> GPSSRWSKDYDVCVCHSEEDLVAAQDLVSYLEGSTASLRCFLQLRDATPGGAIVSELCQALSSSHCRVLLITPGFLQDPWCKYQMLQALTE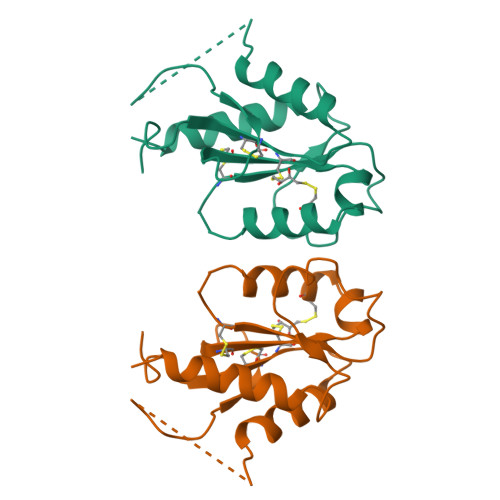APGAEGCTIPLLSGLSRAAYPPELRFMYYVDGRGPDGGFRQVKEAVMRYLQTLS>[2x]MSISISYSTTYSGWTVADYLADWSAYFGDVNHRPGQVVDGSNTGGFN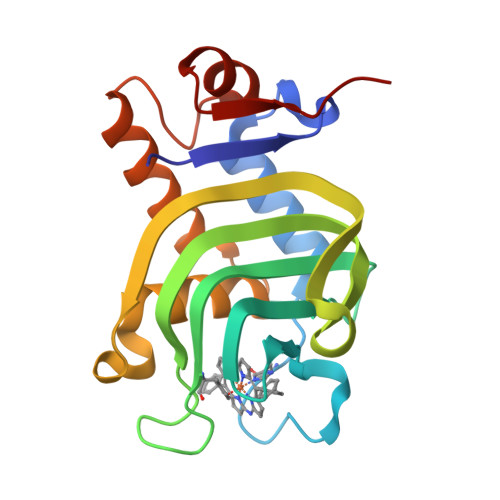PGPFDGSQYALKSTASDAAFIAGGDLHYTLFSNPSHTLWGKLDSIALGDTLTGGASSGGYALDSQEVSFSNLGLDSPIAQGRDGTVHKVVYGLMSGDSSALQGQIDALLKAVDPSLSINSTFDQLAAAGVAHATPAA> ALESLRGNADLAYILSMEPCGHCLIINNVNFCRESGLRTRTGSNIDCEKLRRRFSSLHFMVEVKGDLTAKKMVLALLELARQDHGALDCCVVVILSHGCQASHLQFPGAVYGTDGCPVSVEKIVNIFNGTSCPSLGGKPKLFFIQACGGEQKDHGFEVASTSPEDESPGSNPEPDATPFQEGLRTFDQLDAISSLPTPSDIFVSYSTFPGFVSWRD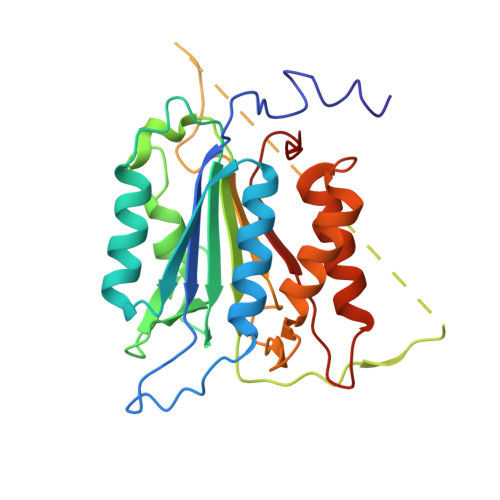PKSGSWYVETLDDIFEQWAHSEDLQSLLLRVANAVSVKGIYKQMPGCFNFLRKKLFFKTS>[2x]SNAMTQLTREQVLELFHQRSSTRYYDPAKKISDEDFECILECGRLSPSSVGSEPWKFLVIQNKTLREKMKSFSWGMMNQLDNCSHLVVILAKKNARY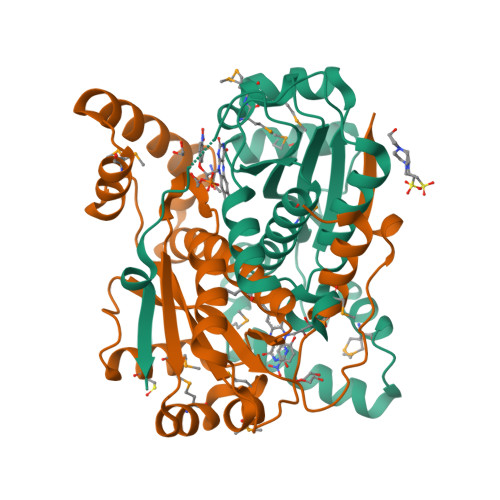DSPFFEDVMVRKGLNAEQQQAALAKYKALQEEDMKLLESDRTLFDWCSKQTYIALANMLTGAAALGIDSCPIEGFHYDKMNECLAEEGLFDPKEYAVSVAATFGYRSRDIAKKSRKALDEVVRWVE I-CreI is a homodimeric member of LHEs family, which recognizes and cleaves a 22 bp pseudo-palindromic target (5′- CAAAACGTCGTGAGACAGTTTG -3′). Each I-CreI monomer binds its own DNA target region generating the catalytic centre at the dimer interface. This region contains two catalytic aspartic acids (D20, one per each monomer). The aspartic side chains participate in the cleavage of the DNA strands along the minor groove, resulting in the hydrolysis of specific phosphodiester bonds upon the coordination of three divalent metal ions.

To decipher why a G at this position restricts cleavage, we made DNA substitutions in the cleavable DNA target to render it non-cleavable. For this purpose, we exchanged GT in positions −5 and −4 of the wild type coding strand target (I-CreI_D75N_target, Fig. 1b upper sequence) by TG, generating the non-cleavable target I-CreI_D75N_target-null (Fig. 1b bottom sequence). The absence of the central metal ion in the non-cleaved structures, would explain the different catalytic behaviour. To assess unambiguously the number of catalytic ions present in the active site, we solved the crystal structure of the two proteins in complex with both target DNAs in the presence of Mn2+, which allows catalysis and unambiguous detection and location through its anomalous diffraction signal. In addition, Mn2+ is less restrictive than Mg2+17 allowing phosphoryl transfer reactions in non-ideal substrates, including the non-cleavable targets studied here. In-depth analysis showed differences in the occupancy of the central metal at the active site between cleavable and non-cleavable targets. A high occupancy level of the central metal ion is essential for the cleavage, and the lower occupancy level of the central Mn2+ ion found in the non-cleavable targets (46% and 74% for I-CreI_D75N_target-null and I-CreI_3115_target-null, respectively) compared with the cleavable ones (100% in both cases) revealed that the non-cleavable targets interfere with the positioning of the central metal ion affecting catalysis. Our results clearly point out that in the cases of I-CreI_D75N_target-null and I-CreI_3115_target-null sequences bound to the I-CreI_D75N and I-CreI_3115 proteins, A at position +1 largely deviates with respect to the usual B-DNA conformation. In particular, we found that in ~ 30% (I-CreI_D75N_target-null) and ~ 60% (I-CreI_3115_target-null) of the simulation time A +1 is not paired and is found stacked to the corresponding nucleobases. The larger flexibility of the A +1 in the active centre explains the low occupancy of the central metal ion within the active site, disturbing the positioning of the P-O bond for catalysis, thus inhibiting cleavage.

>[2x]NTKYNKEFLLYLAGFVDGDGSIIAQIKPNQSYKFKHQLSLTFQVTQKTQRRWFLDKLVDEIGVGYVRDRGSVSNYILSEIKPLHNFLTQLQPFLKLKQKQANLVLKIIEQLPSAKESPDKFLEVCTWVDQIAALNDSKTRKTTSETVRAVLDAA> GSSPQREPQRVSHEQFRAALQLVVDPGDPRSYLDNFIKIGEGSTGIVCIATVRSSGKLVAVKKMDLRKQQRRELLFNEVVIMRDYQHENVVEMYNSYLVGDELWVVMEFLEGGALTDIVTHTRMNEEQIAAVCLAVLQALSVLHAQGVIHRDIKSDSILLTHDGRVKLSDFGFCAQVSKEVPRRKSLVGTPYWMAPELISRLPYGPEVDIWSLGIMVIEMVDGEPPYFNEPPLKAMKMIRDNLPPRLKNLHKVSPSLKGFLDRLLVRDPAQRATAAELLKHPFLAKAGPPASIVPLMRQNRTR

PAKs are serine/threonine protein kinases that are regulated by Rho GTPases of the Cdc42 and Rac families (Knaus et al., 1995; Manser et al., 1994; Martin et al., 1995). In humans, the PAK family comprises six members, which are classified into groups I (PAK1, -2, and -3) and II (PAK4, -5, and -6) based on their domain architecture and regulatory properties (Bokoch, 2003; Jaffer and Chernoff, 2002; Kumar et al., 2006; Zhao and Manser, 2005). Group II PAKs (PAK4–6) regulate a wide variety of cellular functions, and PAK deregulation has been linked to tumor development. Comparison of five high-resolution crystal structures comprising the kinase domains of all three monophosphorylated, enzymatically active group II PAK family members revealed a number of catalytically productive and nonproductive conformers presumably representing snapshots of catalytic domain movements during catalysis.

In order to elucidate the molecular mechanisms of inhibition, we determined the structures of a 2, 6, 9-trisubstituted purine inhibitor (N-(cis-2-Aminocyclohexyl)-N-(3-chlorophenyl)-9-ethyl-9H-purine-2, 6-diamine) with PAK4 and PAK5. The 2, 6, 9-trisubstituted purine inhibitor (CGP74514A) has been described as a potent and cell-permeable inhibitor of Cdk1/cyclin B (Giocanti et al., 1999; Wang et al., 2003). To shed light on this conformational plasticity of group II PAKs, we identified small-molecule inhibitors and used them to trap the kinase domains in their closed conformations. Binding of adenine-mimetic inhibitors to the active sites of PAK4 and PAK5 resulted in the expected clamping movement of the two kinase lobes and closure of the active site, as will be described below. In PAK4 and PAK5, the inhibitor interacted with conserved active site residues. The binding orientations of the purine scaffold in PAK4 and PAK5 differed slightly; however, the mode of binding was identical to the one observed in the Src kinase complex (Dalgarno et al., 2006). As an example, the interactions of the inhibitor and the PAK4 kinase domain are described. In PAK4, and in the analogous residues in PAK5, the inhibitor forms two hydrogen bonds with the hinge backbone residue Leu398. In addition, several hydrophobic interactions with the active site residues Phe397, Ile327, Ala348, and Val335 in the N-terminal kinase lobe and Leu398, Leu447, Gly401 and Val379 in the C-terminal kinase lobe are present. Similar rearrangements of helix αC were also observed when the PAK4 inhibitor complex was compared with PAK4Etgly, suggesting that this novel, to our knowledge, mechanism is conserved in group II PAKs (not shown). In the PAK4EtGly structure, the corresponding arginine (Arg359) forms hydrogen bonds with the phosphate moiety of the phosphorylated activation loop residue S474; in the PAK4 purine complex, Arg359 forms an indirect interaction with that residue via a sulfate ion present in the crystallization solution.> GPQDNPYERGPDPTEDSIEAIRGPFSVATERVSSFASGFGGGTIYYPRETDEGTFGAVAVAPGFTASQGSMSWYG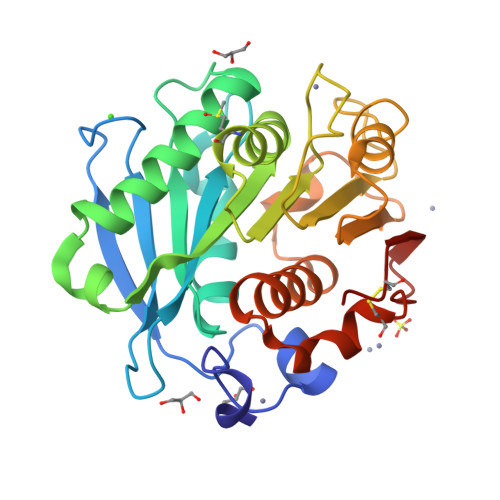ERVASQGFIVFTIDTNTRLDQPGQRGRQLLAALDYLVERSDRKVRERLDPNRLAVMGHAMGGGGSLEATVMRPSLKASIPLTPWNLDKTWGQVQVPTFIIGAELDTIAPVSTHAKPFYESLPSSLPKAYMELDGATHFAPNIPNTTIAKYVISWLKRFVDEDTRYSQFLCPNPTDRAIEEYRSTCPYKLN> MARIIVVTSGKGGVGKTTSSAAIATGLAQKGKKTVVIDFAIGLRNLDLIMGCERRVVYDFVNVIQGDATLNQALIKDKRTENLYILPASQTRDKDALTREGVAKVLDDLKAMDFEFIVCDSPAG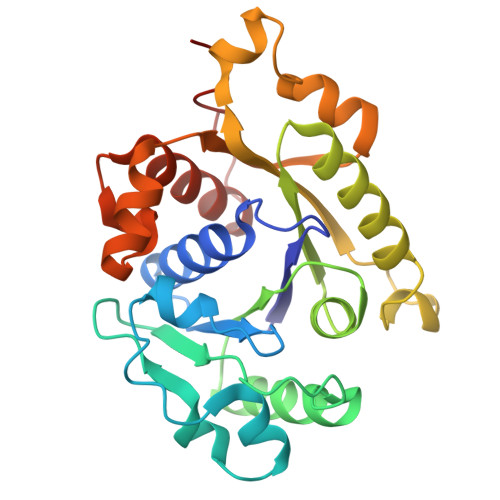IETGALMALYFADEAIITTNPEVSSVRDSDRILGILASKSRRAENGEEPIKEHLLLTRYNPGRVSRGDMLSMEDVLEILRIKLVGVIPEDQSVLRASNQGEPVILDINADAGKAYADTVERLLGEERPFRFIEEEK12-methoxylauric acid | 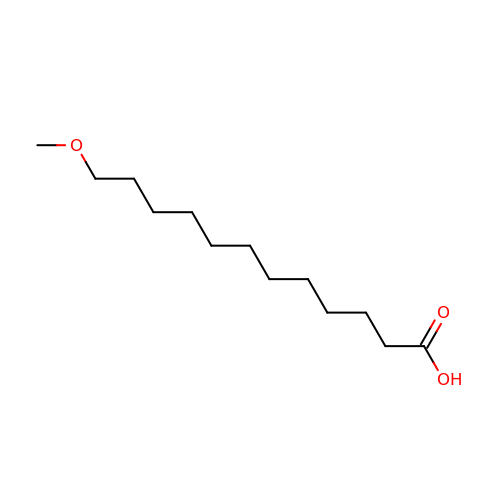C13 H26 O3 | OGLQEYICTWWJQB-UHFFFAOYSA-N>GSGSHVTLPFYPKSPQSKDLIKEAILDNDFMKNLELSQIQEIVDCMYPVEYGKDSCIIKEGDVGSLVYVMEDGKVEV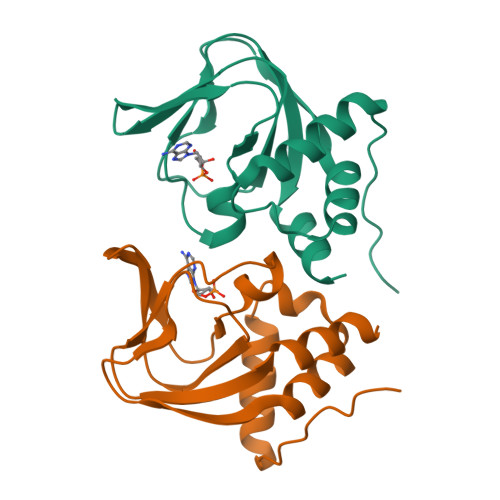TKEGVKLCTMGPGKVFGELAILYNCTRTATVKTLVNVKLWAIDRQCFQTIMMRTGLIKHTEY[2x]> MAGNSGSGAAAAANLNAVRETMDVLLEISRILNTGLDMETLSICVRLCEQGINPEALSSVI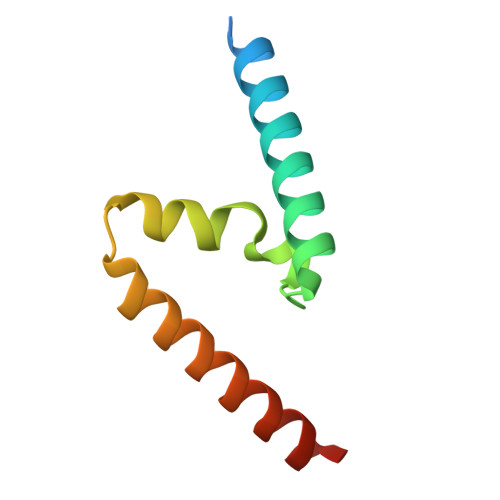KELRKATEALKAAENMTS>LPAGCETAILFPMRSKKIFGSVHPVRPMRLESFSACIWVKATDVLNKTILFSYGTKRNPYEIQLYLSYQSIVFVVGGEENKLVAEAMVSLGRWTHLCGTWNSEEGLTSLWVNGELAATTVEMATGHIVPEGGILQIGQEKNGCCVGGGFDETLAFSGRLTGFNIWDSVLSNEEIRET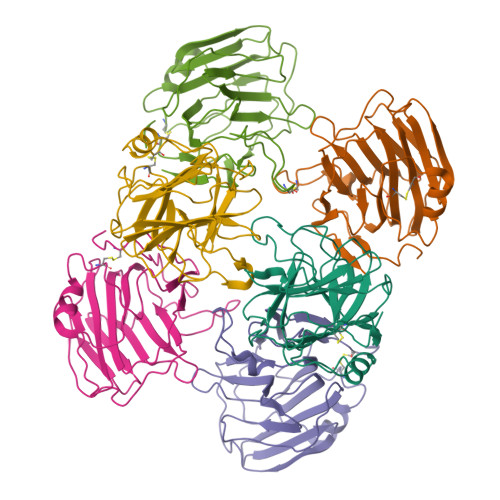GGAESCHIRGNIVGWGVTEIQPHGGAQYVS[6x]7-[3-(aminomethyl)-4-(cyclobutylmethoxy)phenyl]-4-methylquinolin-2-amine 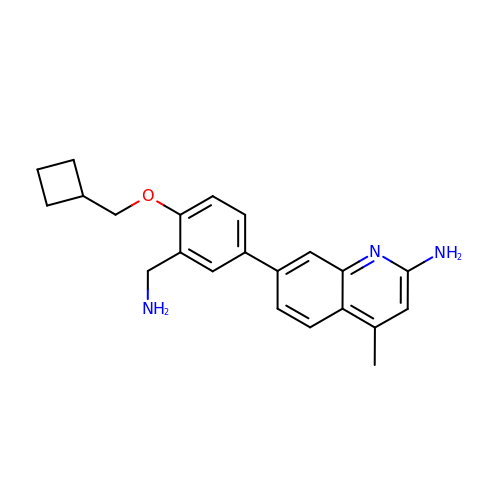| C22 H25 N3 O | COAPMJAWQNAPQG-UHFFFAOYSA-N>[2x]MLEYSELYPIQNEYRMMQSLDGMWKFQFDPEEIGKKSGWENGLPAPVSMPVPSSFADFFTDHKERDYCGDFWYETEFYLPAEWRNKKIWLRFGSITHRGTVYCNGMEITSHEGGFLPVLADISTVAKPGQVNQVVVKINNELNETSLPCGATKILNNGRKLAKPYFDFFNYSGLQRSVWVIALPEESVKDYSVDYELCGTDALVKYEVVTTGEHPVIVRLLDAEGELVA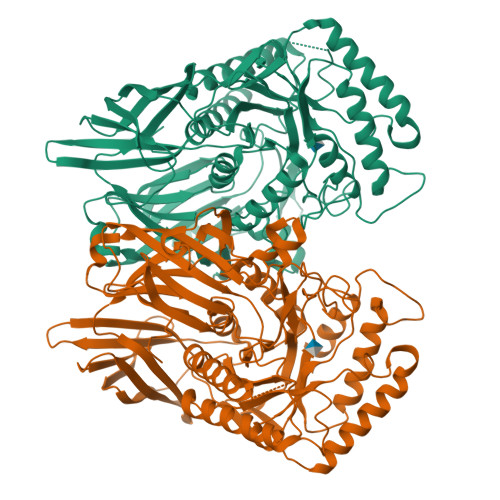ETEGKEGILQVANARLWEVRNAYLYQIVILITDGNGVLDEYREKIGIRTVRIEGTKILLNDRPVYLKGFGKHEDFPILGRGFHWGIVKRDFECLKWTNANCFRTSHYPYAEEWYQFADEEGFLIIDEVPAVGMMRSTRNFVAAGSGNYTYFFEALTVPELLKSHIADTEEMITRDKNHPSVIAWSLFNEPETITDYAYEYFKEVFAAAETYDFQSRPMTGAFEKNSKPELCKCYPLCDFICLNRYYGWYISGGPEIEEAEELFRDEMDRWKAKELNVPFVFTEFGTDTMAGLHKLPSIMWSEEYQKEYLEMNFRVFDSYEFVQGELAWNFADFQTTEGIMRVDGNHKGVFTRDRQPKAAAVVFKDRWEKKNELF> GS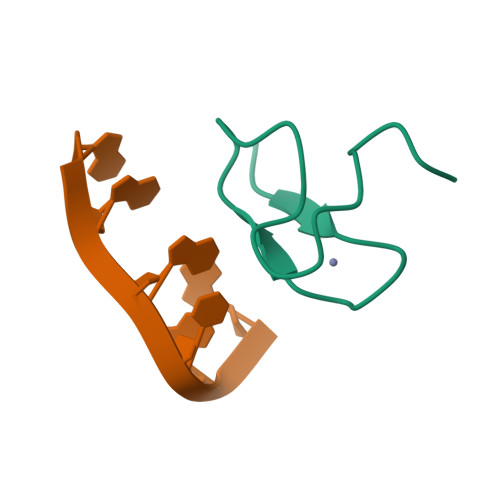SANDWQCKTCSNVNWARRSECNMCNTPKYAK2-[[3-(1,4-diazepan-1-yl)phenyl]amino]-4-[4-methyl-2-(methylamino)-1,3-thiazol-5-yl]pyrimidine-5-carbonitrile 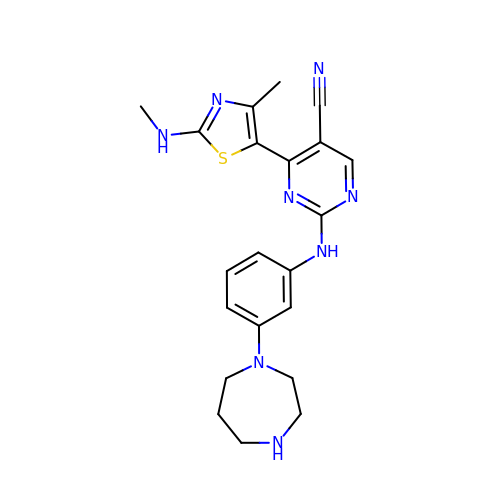| C21 H24 N8 S | BKOYUSKBPMSUBK-UHFFFAOYSA-N> RILPADIKREVLIKDENAETNPDWGFPPEKRPIEMHIQFGVINLDKPPGPTSHEVVAWIKKILNLEKAGHGGTLDPKVSGVLPVALEKATRVVQALLPAGKEYVALMHLHGDVP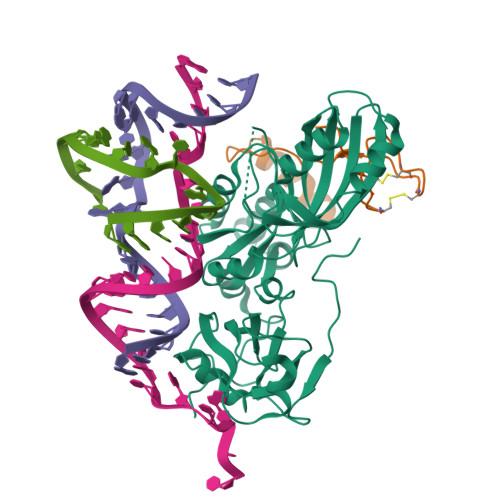EDKIIQVMKEFEGEIIQRPPLRSAVKRRLRTRKVYYIEVLEIEGRDVLFRVGVEAGTYIRSLIHHIGLALGVGAHMSELRRTRSGPFKEDETLITLHDLVDYYYFWKEDGIEEYFRKAIQPMEKAVEHLPKVWIKDSAVAAVTHGADLAVPGIAKLHAGIKRGDLVAIMTLKDELVALGKAMMTSQEMLEKTKGIAVDVEKVFMPRDWYPKLW;> FRIRKCPKCGRYTLKEVCPVCGEKTKVAHPPRFSPEDPYGEYRRRWKREVLGI>MKEDQVVAEEPGFQDEEESLFQDIDLLQKHGINVADIKKLKSVGICTIKGIQMTTRRALCNVKGLSEAKVDKIKEAANKLIEPGFLTAFEYSEKRKMVFHITTGSQEFDKLLGGGIESMAITEAFGEFRTGKTQLSHTLCVTAQLPGAGGYPGGKIIFIDTENTFRPDRLRDIADRFNVDHDAVLDNVLYARAYTSEHQMELLDYVAAKFHEEAGIFKLLIIDSIMALFRVDFSGRGELAERQQKLAQMLSRLQKISEEYNVAVFVTNQMTADPGATMTFQADPKKPIGGHILAHASTTRISLRKGRGELRIAKIYDSPEMPENEATFAITAGGIGDAKE[3x]

During HR, a recombinase binds to single-stranded DNA (ssDNA) and forms a right-handed helical nucleoprotein filament, known as a presynaptic filament, which then searches double-stranded DNA (dsDNA) for homology. Eukaryotic RAD51 and DMC1 both catalyze strand displacement and strand exchange. Interestingly, DMC1 possesses the ability of stabilizing mismatch-containing recombination intermediates (low-fidelity recombinase), whereas the RAD51 lacks the ability to do so (high-fidelity recombinase). RAD51 and DMC1 are members of the RecA family of DNA recombinases and share ~50% amino acid identity and similar biochemical properties.

We then successfully solved the structure of the mismatched dsDNA complex of DMC1 filaments (Structure 3, 3.36 Å). As the binding is not sequence-specific and as there could only be one mismatch in 15 basepairs (Oligo 3/5 with an A–C mismatch in Supplementary Table 2) for obtaining a stable mismatch structure, the densities of basepairs are averaged out in both homologous and mismatched structures. Even though the sidechain of Gln244 in this duet is somewhat far from the phosphodiester (4.4 Å for homologous and 4.2 Å for mismatched DNA) for a direct interaction, its functional role in stabilizing DNA backbone cannot be ruled out considering the moderate resolution of the cryo-EM structures and the change of sidechain orientation in the DMC1-Q244M mutant and WT RAD51. The RMSD values of mismatched DNA are substantially larger than those of homologous DNA for RAD51, but only slightly different for DMC1 and RAD51-VpDg, supporting that DMC1 can stabilize mismatched basepairs. The results taken together support that DMC1 can tolerate mismatched dsDNA by stabilizing not only the basepairs (by providing space for misalignment) but also the DNA backbone, as proposed in the structural model.> MDPPARKEKTKVKESVSRVE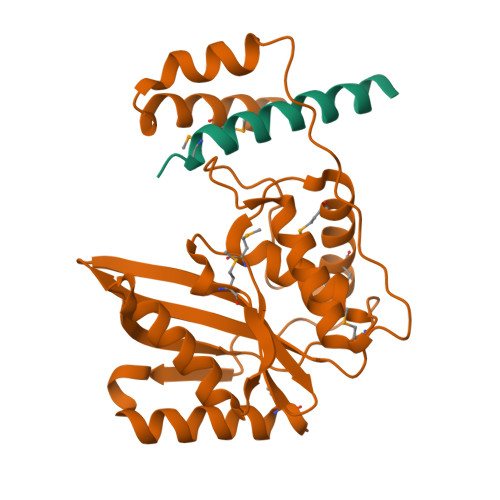KAKQKSAQQELKQRQRAEIYALNRVMTELEQQQFDEFCKQMQPPGE;> MDEATWERMWKHVAKIHPDGEKVAQRIRGATDLPKIPIPSVPTFQPSTPVPERLEAVQRYIRELQYNHTGTQFFEIKKSRPLTGLMDLAKEMTKEALPIKCLEAVILGIYLTNSMPTLERFPISFKTYFSGNYFRHIVLGVNFAGRYGALGMSRREDLMYKPPAFRTLSELVLDFEAAYGRCWHVLKKVKLGQSVSHDPHSVEQIEWKHSVLDVERLGRDDFRKELERHARDMRLKIG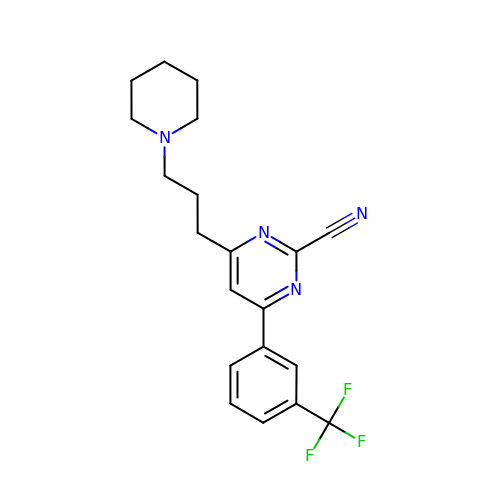4-(3-piperidin-1-ylpropyl)-6-[3-(trifluoromethyl)phenyl]pyrimidine-2-carbonitrile | C20 H21 F3 N4 | XGXDWBUGQKHTSH-UHFFFAOYSA-N> LMSQFEKQKEQGNSLFKQGLYREAVHCYDQLITAQPQNPVGYSNKAMALIKLGEYTQAIQMCQQGLRYTSTAEHVAIRSKLQYRLELAQGAVGSVQIPVVEVDELPEGYDRS;> HKIIEEEAGDPMSILRGRNDDGDDNNDPDDGTLPPLFPIENKISGAKIEEIDKNEIAHRNLKQAPAPAPAPHEQQEDVPEYEVKMKRFKGAAYKLRILIENKAPNSKPDRFSPSYNFAENILYINGKLSIPLPRDIVVNAADIKIFHIRKERTLYIYI;> SRMEEVD

The R2TP complex is found in organisms from yeast to humans, and consists of the AAA+ ATPases Rvb1 and Rvb2 (human: RUVBL1 and RUVBL2), a TPR-containing protein, Tah1 (human: Spagh or RPAP3), and Pih1 (also known as NOP17 and Pih1D1, but referred to as Pih1 henceforth; Kakihara and Houry, 2012; Te et al., 2007). Pih1 is the multipoint scaffold of the R2TP complex, coupling the Rvb1-Rvb2 hetero-dodecamer, the Hsp90 chaperone machinery (via Tah1 in yeast or Spagh/RPAP3 in metazoa), and the TTT (Tel2-Tti1-Tti2) complex implicated in activation and stabilization of PIKKs (Hurov et al., 2010; Kakihara and Houry, 2012). The biological roles ascribed to the R2TP complex are directly associated with its ability to interact with the Hsp90 chaperone system and function as an Hsp90 cochaperone (Boulon et al., 2010; Izumi et al., 2012; Takai et al., 2010). Here we present crystal structures of Hsp90-Tah1-Pih1, Hsp90-Spagh/RPAP3, and Pih1-Tel2 complexes that together define key structural links within the R2TP core in yeast and in animals and reveal how R2TP connects the Hsp90 chaperone system to the TTT complex involved in PIKK activation.

We determined the crystal structure of full-length yeast Tah1, bound to both the C-terminal segment of yeast Pih1264–344 and the C-terminal tail peptide (SRMEEVD) of Hsp90, by single-wavelength anomalous dispersion phasing of crystals grown with selenomethionine-labeled Tah1 (see Experimental Procedures) and refined to 2.2 Å. Consistent with earlier nuclear magnetic resonance studies (Back et al., 2013; Jiménez et al., 2012), the core of Tah1 is a TPR domain, which consists of α helices arranged in a repeating antiparallel right-handed helix topology. Unusually, Tah1-TPR contains five helices rather than the seven found in other structurally characterized Hsp90-binding TPR domains (Morgan et al., 2012; Scheufler et al., 2000; Zhang et al., 2005). The C-terminal 20 residues of Tah1 beyond the end of the fifth α helix of the TPR domain has no coherent structure in the isolated protein in solution (Back et al., 2013; Jiménez et al., 2012), but is fully ordered in the complex crystal structure, and forms the majority of the interaction with Pih1 (see below). The C-terminal domain of Pih1264–344 consists of a seven-stranded β sandwich with the topology of a CS domain—a structural motif also found in Hsp90 cochaperones such as p23/Sba1 (Ali et al., 2006) and Sgt1 (Zhang et al., 2008). The Tah1-Pih1-CS interaction buries ∼2,036 Å2 of molecular surface, which is in the range typically associated with constitutive interactions. Most (∼1,720 Å2) of this surface is buried by the C-terminal segment of Tah1. In the Tah1-Pih1-CS complex, the Hsp90 “tail” peptide binds in an extended groove lined by the helices forming the TPR domain, and interacts with residues from the first, third, and fifth helices.> MSTPGAQEVLFRTGIAAVNSTNHLRVYFQDSHGSIRESL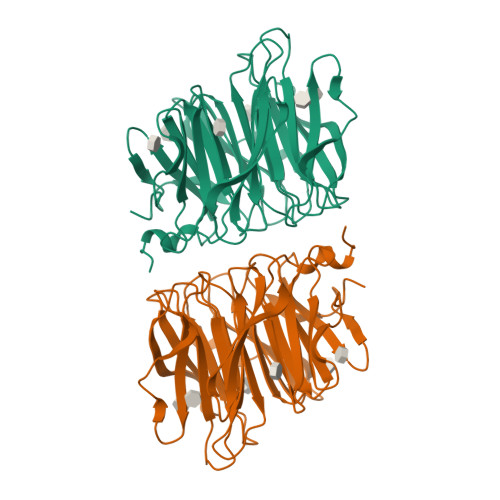YESGWANGTAKNVIAKAKLGTPLAATSKELKNIRVYSLTEDNVLQEAAYDSGSGWYNGALAGAKFTVAPYSRIGSVFLAGTNALQLRIYAQKTDNTIQEYMWNGDGWKEGTNLGVALPGTGIGVTCWRYTDYDGPSIRVWFQTDNLKLVQRAYDPHTGWYKELTTIFDKAPPRCAIAATNFNPGKSSIYMRIYFVNSDNTIWQVCWDHGQGYHDKRTITPVIQGSEIAIISWEGPELRLYFQNGTYVSAISEWTWGKAHGSQLGRRALPPAE>[3x]GPGSMDFRIGQGYDVHQLVPGRPLIIGGVTIPYERGLLGHSDADVLLHAITDALFGAAALGDIGRHFSDTDPRFKG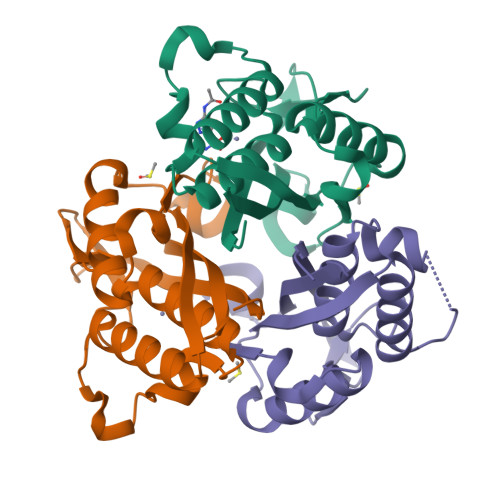ADSRALLRECASRVAQAGFAIRNVDSTIIAQAPKLAPHIDAMRANIAADLDLPLDRVNVKAKTNEKLGYLGRGEGIEAQAAALVVREAAA[(7S)-6-(4-chlorophenyl)-3-(thiophen-2-yl)-7H-[1,2,4]triazolo[3,4-b][1,3,4]thiadiazin-7-yl]acetic acid | C16 H11 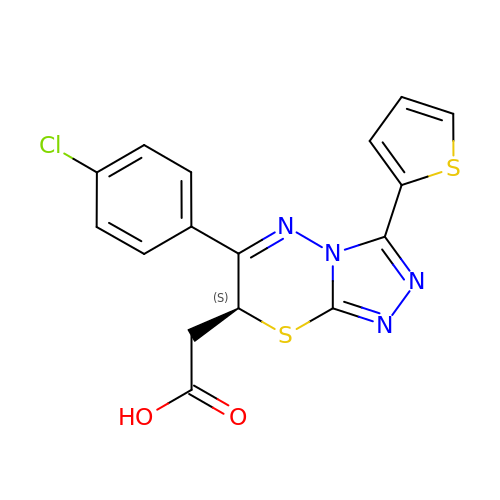Cl N4 O2 S2 | PIDZXRXAOSMZRQ-LBPRGKRZSA-N>ASVASSPQKQHSPKTSGVKSGEEVRIAVLGASGYTGAEIVRLLANHPQFRIKVMTADRKAGEQFGSVFPHLITQDLPNLVAVKDADFSNVDAVFCCLPHGTTQEIIKGLPQELKIVDLSADFRLRDINEYAEWYGHSHRAPELQQEAVYGLTEVLRNEIRNARLVANPGCYPTSIQLPLVPLIKAKLIKVSNIIIDAKSGVSGAGRGAKEANLYTEIAEGIHAYGIKGHRHVPEIEQGLSEAAESKVTI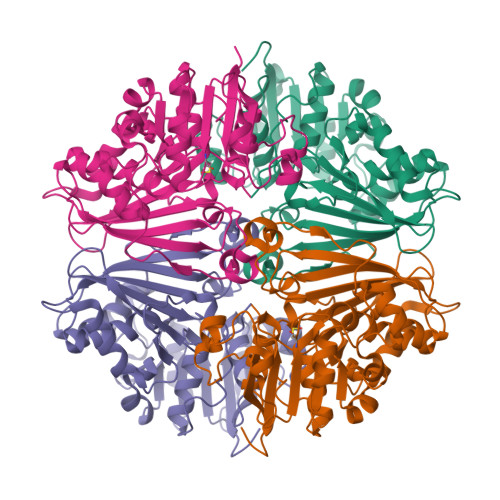SFTPNLICMKRGMQSTMFVEMAPGVTANDLYQHLKSTYEGEEFVKLLNGSSVPHTRHVVGSNYCFMNVFEDRIPGRAIIISVIDNLVKGASGQAVQNLNLMMGLPENTGLQYQPLFP[4x]> AMVSMKEFIGRWKLVHSENFEEYLKEIGVGLLIRKAASLTSPTLEIKLDGDTWHFNQYSTFKNNKLAFKIREKFVEIAPDERSYNTLVTFENGKFISHQDKIKENHHSSVFTTWLENGKLLQTYQSGSVICRREFVKE

Folick et al. further identified a Lipid Binding Protein 8 (LBP-8) that mediates the retrograde signaling between lysosomal lipid hydrolysis and nuclear transcription. LBP-8 is a member of a larger family of proteins termed the intracellular lipid-binding proteins (iLBPs), which includes both fatty acid binding proteins (FABPs), cellular retinoic acid binding proteins (CRABPs), and cellular retinoid binding proteins (CRBPs). Interestingly, LBP-8 itself is also sufficient to prolong lifespan through activating NHR-49 and NHR-808. Here, we have expanded our knowledge of the FABP family by reporting the first structure of a C. elegans FABP, LBP-8, and exploring its ligand specificity.

The LBP-8 structure was solved in the C121 space group at high resolution (1.3 Å), with the asymmetric unit containing a monomer, which was consistent with size exclusion chromatography. The crystal structure includes all 137 amino acids of wild type LBP-8, 92 waters, and two sulfate anions. LBP-8 adopts a typical lipocalin fold, present in all FABPs, consisting of a N-terminal alpha helix-turn-helix motif lid (αA- αB) and a twisted beta barrel containing ten antiparallel strands (βA-βJ). The interior cavity is lined with polar and hydrophobic residues generating a solvent accessible surface area of 825 Å2 and volume of 1170 Å3. There are fragments of continuous electron density present throughout the pocket; however, we were unable to model in a fatty acid with confidence. We do predict that fatty acid is binding to LBP-8 based on lipid MS data, therefore, the fragmented electron density likely reflects that only a fraction of the LBP-8 in the crystal bound to fatty acid, or the fatty acid does not adopt a preferred conformation in the pocket. A network of eleven waters are present in the putative lipid binding pocket and anchored via hydrogen bonds with amino acids glutamine 56 and arginine 132. The LBP-8 structure contains two lysines (K24 and K34) and an arginine (R33) present in the alpha helical lid, and a hydrophobic patch (25-IGVGLLI-32) within the turn region, suggesting LBP-8 is a “collisional” FABP, and directly interacts with membranes or membrane proteins to acquire fatty acids. The interior cavity of LBP-8 is lined with hydrophobic residues (F19, F60, L65, F67, F73, F94, F110, T112, and F134), which can stabilize fatty acyl tails of fatty acids via hydrophobic interactions. The absence of these conserved amino acids and having large pocket volume suggest that fatty acids can bind variably, possibly explaining why there was such diversity in our lipid MS data and disordered electron density within the interior of the crystal structure.> SIDGGIRAATSQEINELTYYTTLSANSYCRTVIPGATWDCIHCDATEDLKIIKTWSTLIYDTNAMVARGDSEKTIYIVFRGSSSIRNWIADLTFVPVSYPPVSGTKVHKGFLDSYGEVQNELVATVLDQFKQYPSYKVAVTGHSLGGATALLCALDLYQREEGLSSSNLFLYTQGQPRVGNPAFANYVVSTGIPYRRTVNERDIVPHLPPAAFGFLHAGSEYWITDNSPETVQVCTSDLETSD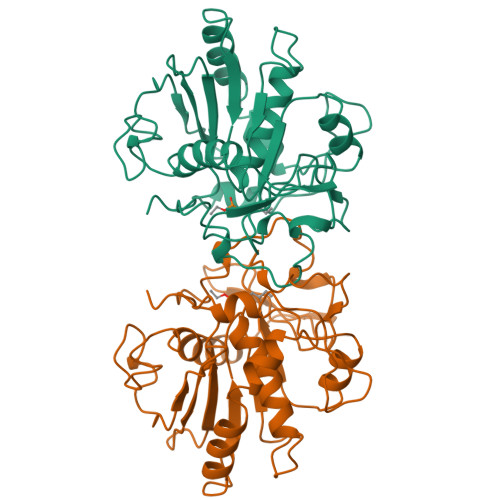CSNSIVPFTSVLDHLSYFGINTGLCT> SMHSDLTFCEIILMEMES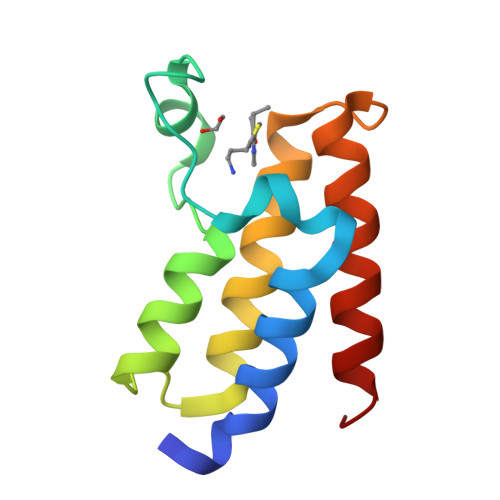HDAAWPFLEPVNPRLVSGYRRIIKNPMDFSTMRHRLSRGGYTSSEEFAADALLVFDNCQTFNEDDSEVGKAGHIMRRFFESRWEEFY>MSLLAKIVDGKNLSFEEAYELFNELKGSDGVLIGAYLAALQTKGYTGEELAGLARAMRDSAVKLDLGKVADTAGTGGDGSSTINVSTASALILSAFTRVAKHGNVSITSKSGSANVLEALGLNIRVSPERAREMVESTNFTFIFAPAYHPALRPIMPVRKALGIKTVFNVIGPLANPADPAYQVVGVNSPELLEPVAEALEFLGVERALVVHGSGMDEVSPHRETLVLEVGNGVERYTLSPEDFGIEPVKPLPCSSPEESAARIKAVLGGSGRREDRDFILVNASAALYASGVAEDFREGLEMA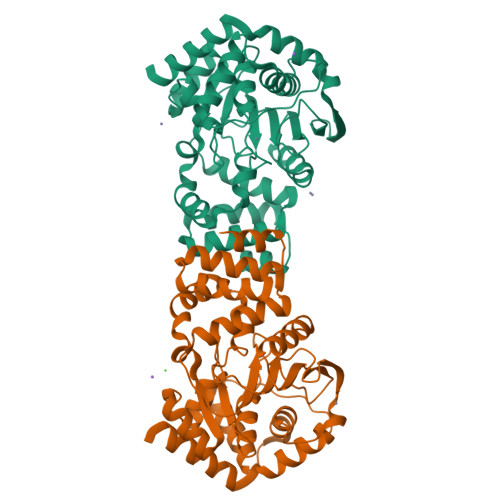REALGQGMLEKLEEIACLSKS[2x]> MERLQPGVTLTESIITMGQQEIPSAVPVFIGYTVRYPEQSEASVRIDSLAEYTSLFGDDHVMMFAVRHYFDNGGQQAFVLPLKDNMPSVEMTTAEAENLIAALRSATVSEAIGGHSQITLILVPDMARLNDSDIDDSSTQVSLWSQGWEALLQLSQVRPNLFVLLDAPDNVEQAQKCMTTLSSDYRQWGAAYWPRLETTYQKEISGKDNESQGIFQGTVLSPTAAVAAVIQRTDNDAGVWKAPANIALSQVIRPVKSYLQGSVLFNSSGTSLNVIRSFPGKGIRVWGCRTLENTDNTQWRYLQTRRLVSYVTAHLTQLARMYVFEPNNELTWMKLKGQSYNWLRQLWLQG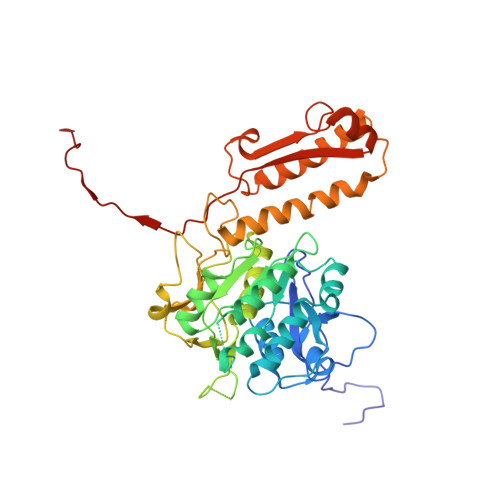GLYGSQEDEAFNILLGVNETMTEDDVRAGKMIMKVELAVLFPAEFIEISLVFNTQTEALS>[2x]HHHHHHSSGLVPRGSMTATETVRVRFCPSPTGTPHVGLVRTALFNWAYARHTGGTFVFRIEDTDAQRDSEESYLALLDALRWLGLDWDEGPEVGGPYGPYRQSQRAEIYRDVLARLLAAGEAYHAFS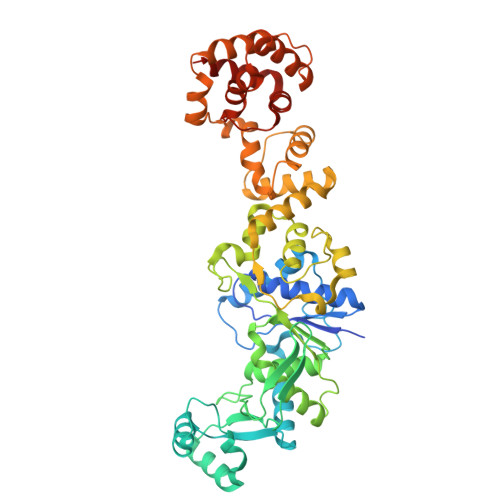TPEEVEARHVAAGRNPKLGYDNFDRHLTDAQRAAYLAEGRQPVVRLRMPDDDLAWNDLVRGPVTFAAGSVPDFALTRASGDPLYTLVNPCDDALMKITHVLRGEDLLPSTPRQLALHQALIRIGVAERIPKFAHLPTVLGEGTKKLSKRDPQSNLFAHRDRGFIPEGLLNYLALLGWSIADDHDLFGLDEMVAAFDVADVNSSPARFDQKKADALNAEHIRMLDVGDFTVRLRDHLDTHGHHIALDEAAFAAAAELMQTRIVVLGDAWELLKFFNDDQYVIDPKAAAKELGPDGAAVLDAALAALTSVTDWTAPLIEAALKDALIEGLALKPRKAFSPIRVAATGTTVSPPLFESLELLGRDRSMQRLRAARQLVGHA>[10x]MTEAQAIAKQLGGVKPDDEWLQAEIARLKGKSIVPLQQVKTLHDWLDGKRKARKSCRVVGESRTGKTVACDAYRYRHKPQQEAGRPPTVPVVYIRPHQKCGPKDLFKKITEYLKYRVTKGTVSDFRDRTIEVLKGCGVEMLIIDEADRLKPETFADVRDIAEDLGIAVVLVGTDRLDAVIKRDEQVLERFRAHLRFGKLSGEDFKNTVEMWEQMVLKLPVSSNLKSKEMLRILTSATEGYIGRLDEILREAAIRSLSRGLKKIDKAVLQEVAKEYK;>[10x]IEVWDYEQLREEYGF

pmcCRISPR-associated transposons (CASTs) have co-opted Cas genes for RNA-guided DNA integration and are promising candidates for novel genome-editing methods. Despite remarkable diversity, all RNA-directed transposition systems characterized to date share multiple components: a CRISPR effector (Cas12k or Cascade), proteins dedicated to target capture (TniQ + TnsC), and a transposase called TnsB. By analogy to work from prototypic Tn7 (2), TnsB carries out transposon end recognition, pairing, and the chemical steps which result in integration of cognate element DNA. We determine the molecular mechanism of TnsB recruitment to the target site (via the AAA+ regulator TnsC) and the structural details of the TnsB transposase.

Motivated by the remarkable structural and functional similarities between MuB and ShCAST TnsC, we reasoned that the C-terminal 109 residues of TnsB (spanning domains IIIα and IIIβ, which we refer to as TnsBCTD) are most likely to interact with the TnsC filament. In order to capture a homogeneous “recruitment-like” state, we added TnsBCTD in excess to AMPPNP-bound TnsC, which forms continuous helical filaments on target DNA. The cryo-EM reconstruction of the TnsC filament coated with TnsBCTD revealed side-chain density features (3.5-Å resolution) corresponding to 14 residues decorating the surface of TnsC filaments. Atomic modeling into this density indicated that this portion of TnsB most likely corresponds to the last 15 residues of TnsB (the last residue is not modeled), or residue positions 570 to 584, which we refer to as TnsBHook. The lack of additional density corresponding to TnsBCTD in our cryo-EM reconstruction suggests positions outside the structured TnsBHook do not make specific contacts with the TnsC filament, which is consistent with TnsB disorder predictions. Taken together, the most parsimonious explanation for this is that the TnsBHook represents a structured interaction with TnsC connected by a flexible linker to the rest of the full-length TnsB. Deletions of either the TnsBCTD (ΔCTD, or equivalently TnsBΔCTD, corresponding to residues 1 to 475) or the TnsBHook (ΔHook, or TnsBΔHook, corresponding to residues 1 to 569) result in loss of transposition activity. TnsB’s C-terminal hook interacts with TnsC along the surface of the filament, but interaction via the TnsBHook alone is insufficient to stimulate TnsC filament disassembly, indicating that one or more additional interactions between TnsB and TnsC not visualized here must be required. A total of 50 residues (520 to 569) are not observed in either our TnsBCTD–TnsC structure nor the TnsB STC structure, and are consistent with predictions of disorder based on primary sequence.> PISPIETVPVKLKPGMDGPKVKQWPLTEEKIKALVEICTEMEKEGKISKIGPENPYNTPVFAIKKKNSTRWRKLVDFRELNKRTQDFWEVQLGIPHPAGLKKKKSVTVLDVGDAYFSVPLDEDFRKYTAFTIPSINNETPGIRYQYNVLPQGWKGSPAIFQSSMTKILEPFRKQNPDIVIYQYMDDLYVGSDLEIGQHRTKIEELRQHLLRWGLFTPDQKHQKEPPFLWMGYELHPDKWTVQPIVLPEKDSWTVNDI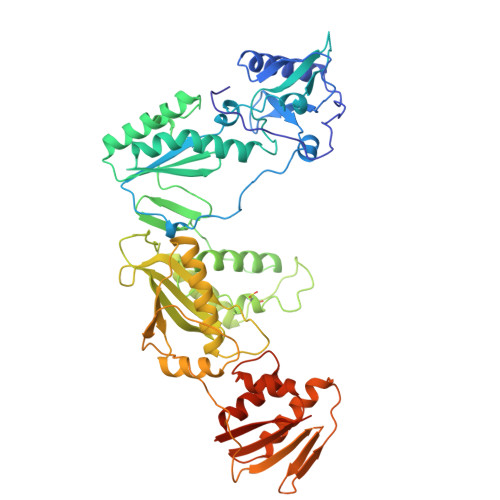QKLVGKLNWASQIYPGIKVRQLCKLLRGTKALTEVIPLTEEAELELAENREILKEPVHGVYYDPSKDLIAEIQKQGQGQWTYQIYQEPFKNLKTGKYARMRGAHTNDVKQLTEAVQKITTESIVIWGKTPKFKLPIQKETWETWWTEYWQATWIPEWEFVNTPPLVKLWYQLEKEPIVGAETFYVDGAANRETKLGKAGYVTNRGRQKVVTLTDTTNQKTELQAIYLALQDSGLEVNIVTDSQYALGIIQAQPDQSESELVNQIIEQLIKKEKVYLAWVPAHKGIGGNEQVDKLVSAGIRKVL(2~{S})-2-azanyl-5-[[(2~{R})-1-(2-hydroxy-2-oxoethylamino)-1-oxidanylidene-3-[(1~{R})-3-oxidanylidene-1-phenyl-propyl]sulfanyl-propan-2-yl]amino]-5-oxidanylidene-pentanoic 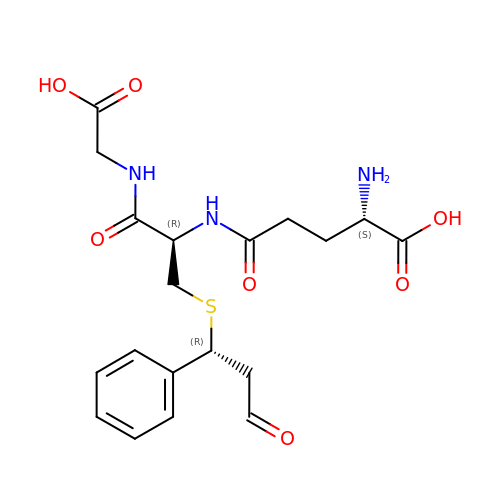acid | C19 H25 N3 O7 S | OOFSDLPAAPKBNR-SOUVJXGZSA-N> GSHMASMNSEILNNIILNLRYKDNNLIDLSGYGAKVEVYDGVELNDKNQFKLTSSANSKIRVTQNQNIIFNSVFLDFSVSFWIRIPKYKNDGIQNYIHNEYTIINCMKNNSGWKISIRGNRIIWTLIDINGKTKSVFFEYNIREDISEYINRWFFVTITNNLNNAKIYINGKLESNTDIKDIREVIANGEIIFKLDGDIDRTQFIWMKYFSIFNTELSQSNIEERYKIQSYSEYLKDFWGNPLMYNKEYYMFNAGNKNSYIKLKKDSPVGEILTRSKYNQNSKYINYRDLYIGEKFIIRRKSNSQSINDDIVRKEDYIYLDFFNLNQEWRVYTYKYFKKEEEKLFLAPISDSDEFYNTIQIKEYDEQPTYSCQLLFKKDEESTDEIGLIGIHRFYESGWWFEEYKDYFCISKWYLKEVKRKPYNLKLGCNWQFIPKDEGWTE;> GEGKEDAFSKLKEKFMNELHK

Botulinum neurotoxins (BoNTs) are a family of protein toxins produced by various clostridial bacteria. BoNTs target motor nerve terminals by binding to specific receptors and enter neurons via receptor-mediated endocytosis. Besides gangliosides, BoNT/B, DC, and G utilize the synaptic vesicle membrane proteins synaptotagmin (Syt) I and II as their protein receptors, whereas BoNT/A, E, and D utilize synaptic vesicle protein 2 (SV2), another family of synaptic vesicle membrane proteins. When BoNT/B was modeled onto cell membranes via anchoring by gangliosides and Syt I/II, an extended loop between its GBS and Syt-binding site was recognized to be at a location ideal for membrane interactions.

We next examined the effect of replacing the tip residues I and V with aromatic ones, including I1248W (designated HC/BW) and a double mutation (I1248W/V1249W, designated HC/BWW). Crystals were successfully obtained for HC/BWW in the presence of the GD1a oligosaccharide and a peptide corresponding to human Syt I (residues 33–53, hSyt I). The structure was solved to a 2.4-Å resolution. The overall structure of HC/BWW is virtually identical to that of WT HC/B. The interactions of HC/BWW with GD1a and hSyt I also match the previously solved structure of HC/B in complex with GD1a and rat Syt II peptides. Recognition of GD1a is based on a stacking interaction between W1262 and the central galactose-4 moiety of the carbohydrate, with the surrounding pocket (including E1190, H1241, S1260, Y1263, and E1273) offering multiple hydrogen bonds to the adjacent N-acetylglucosamine (GalNAc3) and sialic acid group (Sia5). On the other side of the LBL, the Syt peptide occupies the binding crevice and mostly involves hydrophobic interactions. The LBL was clearly defined in the HC/BWW structure and is located between the GBS and Syt-binding site. The loop protrudes significantly, with the side chains of W1248 and W1249 exposed toward the surface at the tip of LBL in HC/BWW. The ternary complex of HC/BWW with both gangliosides and Syt I peptide demonstrates conclusively that introducing two consecutive tryptophan residues does not alter the conformation of HC/B or affect the GBS and Syt-binding site.> EIPLKYGATNEGKRQDPAMQKFRDNRLGAFIHWGLYAIPGGEWNGKVYGGAAEWLKSWAKVPADEWLKLMDQWNPTKFDAKKWAKMAKEMGTKYVKITTKHHEGFCLWPSKYTKYTVANTPYKRDILGELVKAYNDEGIDVHFYFSVMDWSNPDYRYDIKSKEDSIAFSRFLEFTDNQLKELATRYPTVKDFWFDGTWDASVKKNGWWTAHAEQMLKELVPGVAINSRLRADDKGKRHFDSNGRLMGDYESGYERRLPDPVKDLKVTQWDWEACMTIPENQWGYHKDWSLSYVKTPIEVIDRIVHAVSMGGNMVVNFGPQADGDFRPEEKAMATAIGKWMNRYGKAVYACDYAGFEKQDWGYYTRGKNDEVYMVVFNQPYSERLIVKTPKGITVEKATLLTTGEDITVVETTRNEYNVSVPKKNPGEPYVI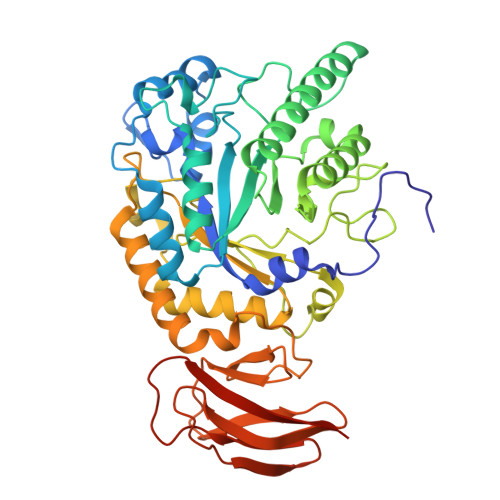QLKVRAAKGTKSIYRDALT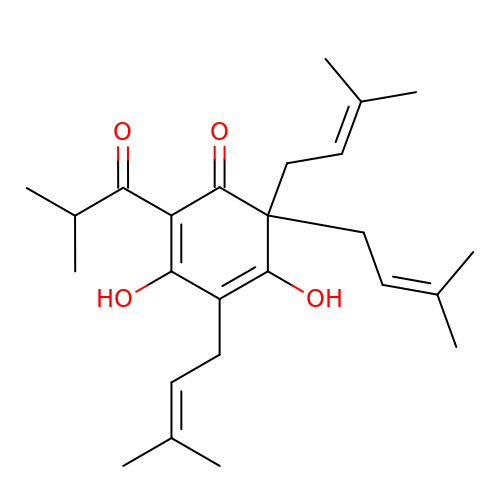3,5-dihydroxy-4,6,6-tris(3-methylbut-2-en-1-yl)-2-(2-methylpropanoyl)cyclohexa-2,4-dien-1-one | C25 H36 O4 | UNCDMWKTFLUPHZ-UHFFFAOYSA-N>MGSSHHHHHHSQDPMTDSTTHYTRPDVAAFLAFLNAQEGPKMEEMPPAGAREMMRVMGQLADVPRGEIAKVEDRMIPGPDGDIPIRLYDNRPDREAGPVMVFYHGGGWVIGDLETHDPYCAEAARILDMPVIAIDYRLAPEHPFPAAPIDCEAATRWV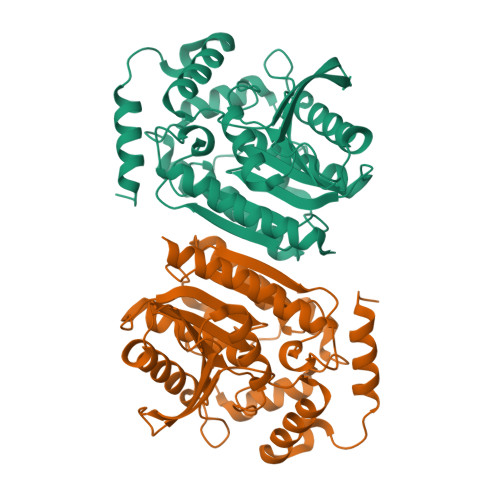ADNIACTGLVLSGDSAGGNLTIVTALALRDEPAAKPVIAIHPIYPAVTTHNDWQSYRDFGEGHLLTEGSMTWFGNHYAADPADRRAAPIDFPADGLPPTLLITASLDPLRDQGRAYAAKLIEAGVPTTYREAKGTIHGYICLAQGIPSAKDDIRGALTVLKAIVAEATGAA[2x]Macrophage Migration Inhibitory Factor (MIF) is a ubiquitous multifunctional protein and a key player in the inflammatory response and innate immunity. MIF has two enzymatic activities: an evolutionarily well conserved keto-enol tautomerase activity and a thiol-protein oxido-reductase activity that is mediated by the C56ALC59 motif. X-ray structural studies have consistently shown that MIF exists as a homotrimer. Each MIF monomer consists of 114 amino acids and is composed of two anti-parallel α-helices packed against a four-stranded β-sheet.

To elucidate the role of intersubunit interactions involving Leu46 on the structure and stability of MIF, we compared the structural stability, and biophysical properties of wt, L46A, L46F and L46G mutants at the secondary, tertiary and quaternary structure levels. To understand the role of Leu46 mutations on the three-dimensional structure of MIF, we also determined the crystal structures of L46F, L46A and L46G huMIF at 1.70 Å, 1.70 Å and 1.60 Å, respectively. Similar to the wild type species, Leu46 mutants crystallized as homotrimeric proteins with dimensions of approximately 35 Å×50 Å×50 Å. In agreement with our previous structural studies, X-ray crystal structures of MIF variants demonstrate that the Leu46 mutants conserve the same three-dimensional structure pattern as the wt protein. Static light scattering, in agreement with the analytical ultracentrifugation data, demonstrated that wt, L46F, L46A and L46G exist as stable trimers. Finally, crystallographic data and enzymatic assays do not show any drastic conformational change of the catalytic site or activity of MIF upon Leu46 mutations. Using hydroxyphenylpyruvate as a substrate, we showed that all Leu46 mutants are enzymatically active. In our case, chemical shift measurements demonstrate an extremely high similarity between L46A and L46G huMIF, whereas the L46F mutant exhibits a slightly different chemical shift pattern. Thus, decreasing the hydrophobicity of residue 46 (via mutations L46A and L46G) destabilizes the hydrophobic pocket and results in distant structural perturbation that is transmitted through the backbone, affecting the tertiary structure of the MIF. Taken together, our data suggest that the intersubunit interactions involving the residue Leu46 play a key role in the structural stability of MIF and provide new insights into the role of a novel intersubunit hydrophobic pocket in modulating MIF’s conformation, stability, and potentially its receptor binding and biological activity.

>[3x]PMFIVNTNVPRASVPDGFLSELTQQLAQATGKPPQYIAVHVVPDQAMAFGGSSEPCALCSLHSIGKIGGAQNRSYSKLLCGLLAERLRISPDRVYINYYDMNAANVGWNNSTFA> AAPGKPTIAWGNTKFAIVEVDQAATAYNNLVKVKNAADVSVSWNLWNGDTGTTAKVLLNGKEAWSGPSTGSSGTANFKVNKGGRYQMQVALCNADGCTASDATEIVVADTDGSHLAPLKEPLLEKNKPYKQNSGKVVGSYFVEWGVYGRNFTVDKIPAQNLTHLLYGFI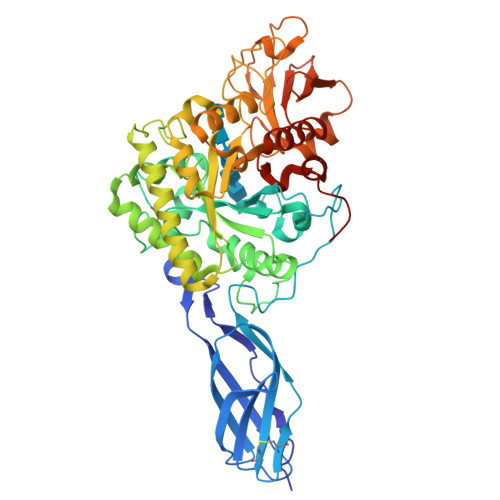PICGGNGINDSLKEIEGSFQALQRSCQGREDFKVSIHDPFAALQKAQKGVTAWDDPYKGNFGQLMALKQAHPDLKILPSIGGWTLSDPFFFMGDKVKRDRFVGSVKEFLQTWKFFDGVDIDWLFPGGKGANPNLGSPQDGETYVLLMKELRAMLDQLSVETGRKYELTSAISAGKDKIDKVAYNVAQNSMDHIFLMSYDFYGAFDLKNLGHQTALNAPAWKPDTAYTTVNGVNALLAQGVKPGKIVVGTAMYGRGWTGVNGYQNNIPFTGTATGPVKGTWENGIVDYRQIASQFMSGEWQYTYDATAEAPYVFKPSTGDLITFDDARSVQAKGKYVLDKQLGGLFSWEIDADNGDILNSMNASLGNSAGVQ> UCCCAGUCCAC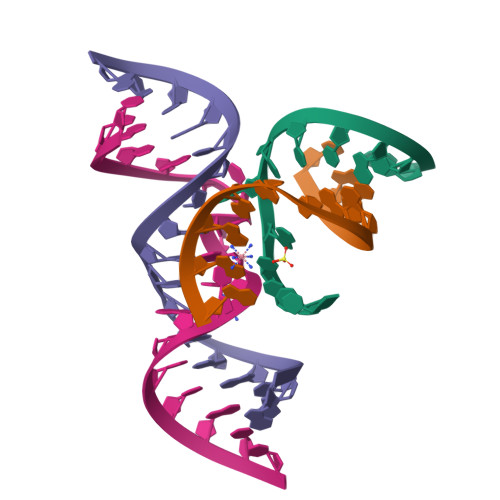CG;> CGGUGAUAAGGG;> GGCAGAGAAACACACGA;> UCGUGGUACAUUACCUGCC> TRKLCSLDNGDCDQFCHEEQNSVVCSCARGYT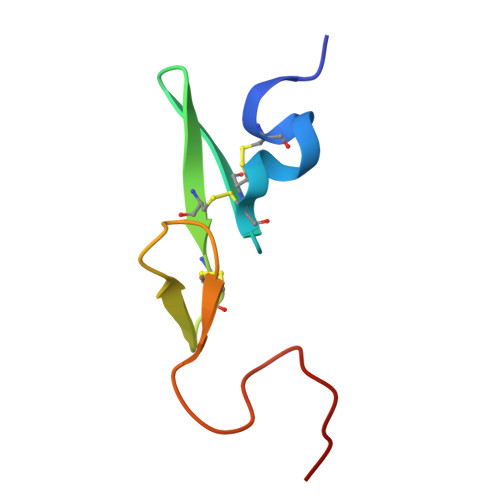LADNGKACIPTGPYPCGKQTLE> MSSMILTQFRPFIESISGITDQSNDVFEDAAKAFSMFTRSDVYKALDEIPFSDDAMLPIPPTIYTKPSHDSYYYIDALNRVRRKTYQGPDDVYVPNCSIVELLEPHETLTSYGRLSEAIENRAKDGDSQARIATTYGRIAESQARQIKAPLEKFVLALLVSEAGGSLYDPVLQKYDEIPDLSHNCPLWCFREICRHISGPLPDRAPYLYLSAGVFWLMSPRMTSAIPPLLSDLVNLAILQQTAGLDPSLVKLGVQICLHAAASSSYAWFILKTKSIFPQNTLHSMYESLEGGYCPNLEWLEPRSDYKFMYMGVMPLSTKYARSAPSNDKKARELGEKYGLSSVVSELRKRTKTYVKHDFASVRYIRDAMACTSGIFLVRTPTETVLQEYTQSPEIKVPIPQKDWTGPVGEIRILKDTTSSIARYLYRTWYLAAARMAAQPRTWDPLFQAIMRSQYVTARGGSGAALRESLYAINVSLPDFKGLPVKAATKIFQAAQLANLPFSHTSVAILADTSMGLRNQVQRRPRSIMPLNVPQQQVSAPHTLTADYINYHMNLSTTSGSAVIEKVIPLGVYASSPPNQSINIDISACDASITWDFFLSVIMAAIHEGVASGSIGKPFMGVPASIVNDESVVGVRAARPISGMQNMIQHLSKLYKRGFSYRVNDSFSPGNDFTHMTTTFPSGSTATSTEHTANNSTMMETFLTVWGPEHTDDPDVLRLMKSLTIQRNYVCQGDDGLMII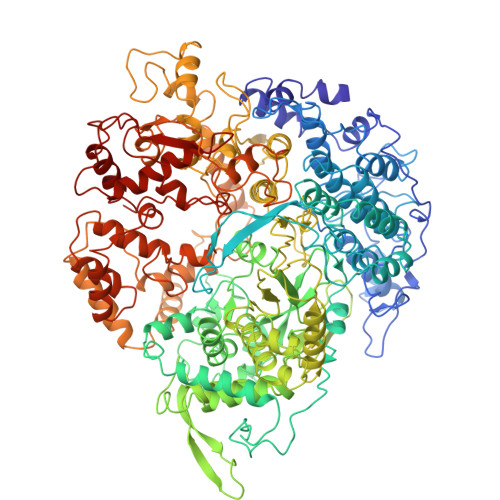DGNTAGKVNSETIQKMLELISKYGEEFGWKYDIAYDGTAEYLKLYFIFGCRIPNLSRHPIVGKERANSSAEEPWPAILDQIMGIFFNGVHDGLQWQRWIRYSWALCCAFSRQRTMIGESVGYLQYPMWSFVYWGLPLVKVFGSDPWIFSWYMPTGDLGMYSWISLIRPLMTRWMVANGYATDRCSPVFGNADYRRCFNEIKLYQGYYMAQLPRNPTKSGRAAPREVREQFTQALSDYLMQNPELKSRVLRGRSEWEKYGAGIIHNPPSLFDVPHKWYLGAQEAATATREELAEMDETLMRARRHSYSSFSKLLEAYLLVKWRMCEAREPSVDLRLPLCAGIDPLNSDPFLKMVSVGPMLQSTRKYFAQTLFMAKTVSGLDVNAIDSALLRLRTLGADKKALTAQLLMVGLQESEADALAGKIMLQDVSTVQLARVVNLAVPDTWMSLDFDSMFKHHVKLLPKDGRHLNTDIPPRMGWLRAILRFLGAGMVMTATGVAVDIYLEDIHGGGRALGQRFMTWMRQEGRSA>[2x]MGSMHAALSTEVVHLRQRTEELLRCNEQQAAELETCKEQLFQSNMERKELHNTVMDLRDNIRVFCRIRPPLESEENRMCCTWTYHDESTVELQSIDAQAKSKMGQQIFSFDQVFHPLSS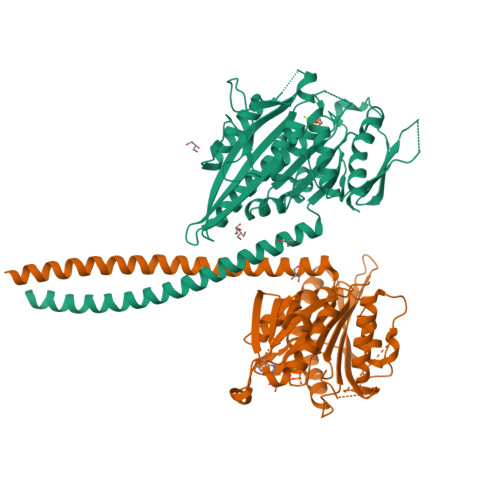QSDIFEMVSPLIQSALDGYNICIFAYGQTGSGKTYTMDGVPESVGVIPRTVDLLFDSIRGYRNLGWEYEIKATFLEIYNEVLYDLLSNEQKDMEIRMAKNNKNDIYVSNITEETVLDPNHLRHLMHTAKMNRATASTAGNERSSRSHAVTKLELIGRHAEKQEISVGSINLVDLAGSESPKTSTRMTETKNINRSLSELTNVILALLQKQDHIPYRNSKLTHLLMPSLGGNSKTLMFINVSPFQDCFQESVKSLRFAASVNSCKMTKAKRNRYLNNSVANSSTQSNNSGSFDK>[4x]MDHHHHHHLP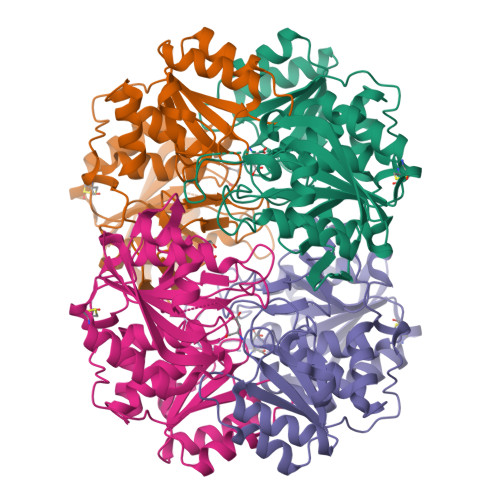NITILATGGTIAGGGDSATKSNYTVGKVGVENLVNAVPQLKDIANVKGEQVVNIGSQDMNDNVWLTLAKKINTDCDKTDGFVITHGVDTMEETAYFLDLTVKCDKPVVMVGAMRPSTSMSADGPFNLYNAVVTAADKASANRGVLVVMNDTVLDGRDVTTTNTTDVATFKSVNYGPLGYIHNGKIDYQRTPARKHTSDTPFDVSKLNELPKVGIVYNYANASDLPAKALVDAGYDGIVSAGVGNGNLYKSVFDTLATAAKTGTAVVRSSRVPTGATTQDAEVDDAKYGFVASGTLNPQKARVLLQLALTQTKDPQQIQQIFNQY>MAALMTPGTGAPPAPGDFSGEGSQGLPDPSPEPKQLPELIRMKRDGGRLSEADIRGFVAAVVNGSAQGAQIGAMLMAIRLRGMDLEETSVLTQALAQSGQQLEWPEAWRQQLVDKHSTGGVGDKVSLVLAPALAACGCKVPMISGRGLGHTGGTLDKLESIPGFNVIQSPEQMQVLLDQAGCCIVGQSEQLVPADGILYAARDVTATVDSLPLITASILSKKLVEGLSALVVDVKFGAGAVFPNQEQARELAKTLVGVGASLGLRVAAALTAMDKPLGRCVGHALEVEEALLCMDGAGPPDLRDLVTTLGGALLWLSGHAGTQAQGAARVAAALDDGSALGRFERMLAAQGVDPGLARALCSGSPAERRQLLPRAREQEELLAPADGTVELVRALPLALVLHELGAGRSRAGEPLRLG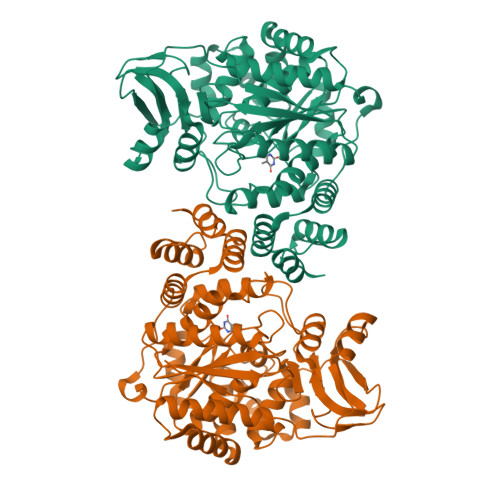VGAELLVDVGQRLRRGTPWLRVHRDGPALSGPQSRALQEALVLSDRAPFAAPLPFAELVLPPQQ[4x]> MASSINPWILTGFADAEGSFLLRIRKNNKSSVGYSTELGFQITLHNKDKSILENIQSTWGVGVIANSGDNAVSLKVTRFEDLKVIIDHFEKYPLITQKYADYMLFKQAFNVMENKEHLTIEGIKELVRIKAKLNWGLTDELKKAFPEIISKERSLINKNIPNFKWLAGFTSGDGCFFVNLIKSKSKLGVQVQLVFSISQHIRDKNLMNSLITYLGCGYIKKKNKSEFSWLEFVVTKFSDI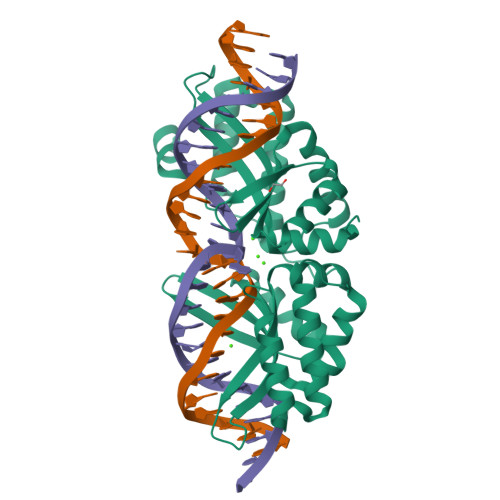RDKIIPFFQEYTLIGTKLKDFEDWCKVAKLIEEKKHLTEEGLDEIKKIKLNMNKGR> ETDEEPEEPGRRGSFVEMVDNLRGKSGQGYYVEMTVGSPPQTLNILVDTGSSNFAVGAAPHPFLHRYYQRQLSSTYRDLRKGVYVPYTQGKWEGELGTDLVSIPHGPNVTVRANIAAITESDKFFINGSNWEGILGLAYAEIARPDDSLEPFFDSLVKQTHVPNLFSLQLCGAGFPLNQSEVLASVGGSMIIGGIDHSLYTGSLWYTPIRREWYYEVIIVRVEINGQDLKMD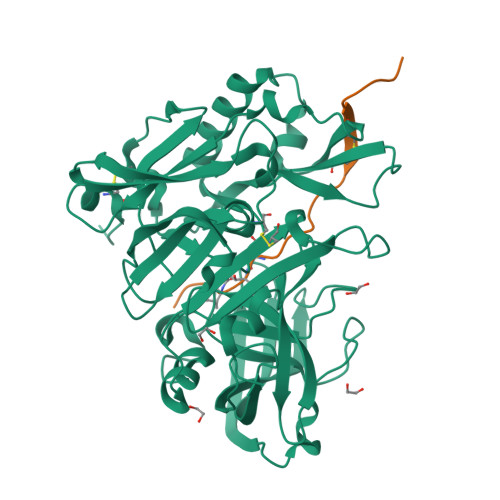CKEYNYDKSIVDSGTTNLRLPKKVFEAAVKSIKAASSTEKFPDGFWLGEQLVCWQAGTTPWNIFPVISLYLMGEVTNQSFRITILPQQYLRPVEDVATSQDDCYKFAISQSSTGTVMGAVIMEGFYVVFDRARKRIGFAVSACHVHDEFRTAAVEGPFVTLDMEDCGYNIPQTDEST;> GGGYPYFIPKGKGEVNXVAEPX>GAMALIEVEKPLYGVEVFVGETAHFEIELSEPDVHG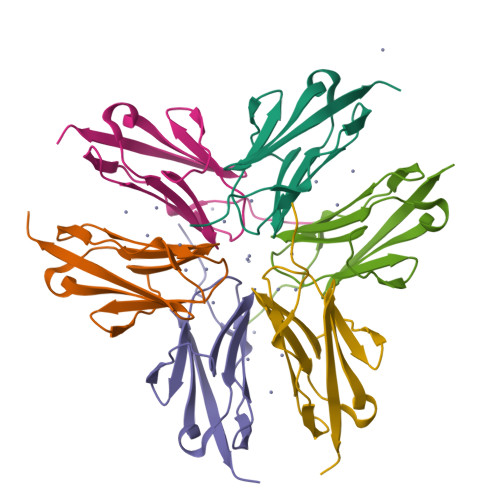QWKLKGQPLAASPDCEIIEDGKKHILILHNCQLGMTGEVSFQAANTKSAANLKVKEL[4x];> GAMALIEVEKPLYGVEVFVGETAHFEIELSEPDVHGQWKLKGQPLAASPDCEIIEEGKKHILILHNCQLGMTGEVSFQAANTKSAANLKVKEL;> GAMALIEVEKPLYGVEVFVGETAHFEIELSEPDVHGQWKLKGQPLAASPDCEIIEDGKKHILILHNCQLGMTGEVSFQAAQTKSAANLKVKEL> PRRRTVGMKSSQGNVPTGNKQ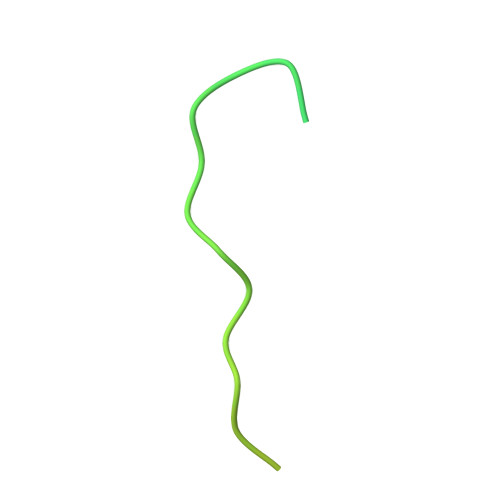SVGKSAKISKPLHIKTSAYQKQYKINLETKARPSAGDEDSAHPDKNKE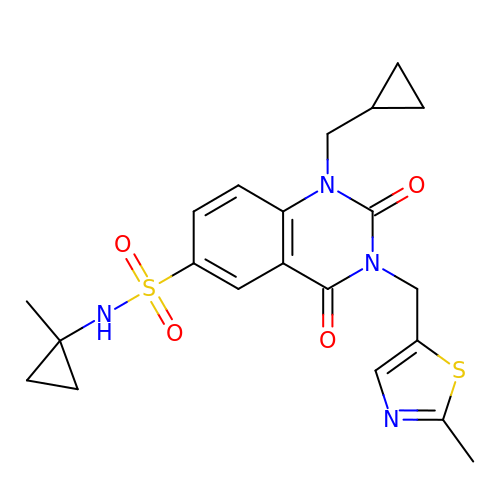1-(cyclopropylmethyl)-6-[[(1-methylcyclopropyl)amino]-bis(oxidanyl)-$l^{4}-sulfanyl]-3-[(2-methyl-1,3-thiazol-5-yl)methyl]quinazoline-2,4-dione | C21 H24 N4 O4 S2 | VHRYOZHNFLYWFP-UHFFFAOYSA-N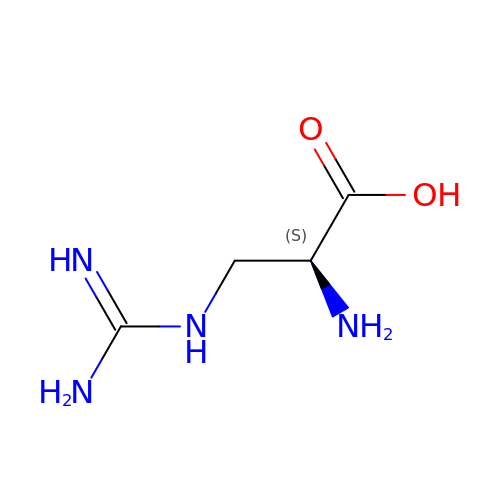2-AMINO-3-GUANIDINO-PROPIONIC ACID | C4 H10 N4 O2 | XNBJHKABANTVCP-REOHCLBHSA-N1-(1-methyl-1H-pyrrol-2-yl)methanamine 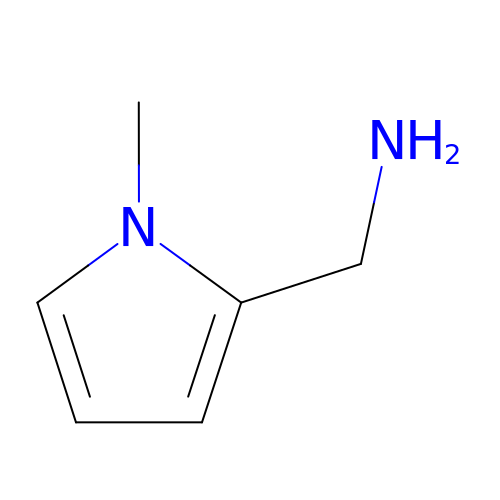| C6 H10 N2 | GGCBARJYVAPZJQ-UHFFFAOYSA-N>NNCPLDWLPMNGLCYKIFNQLKTWEDAEMFCRKYKPGCHLASFHRYGESLEIAEYISDYHKGQENVWIGLRDKKKDFSWEWTDRSCTDYLTWDKNQPDHYQNKEF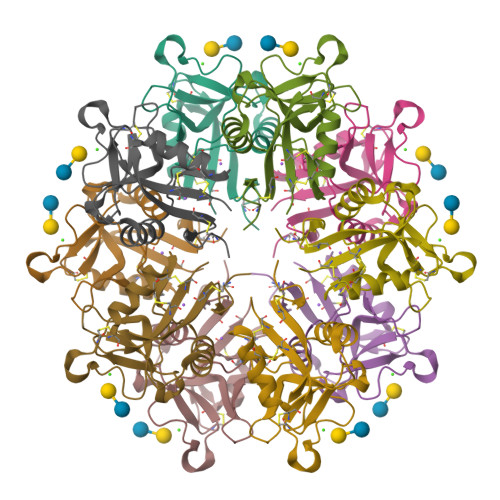CVELVSLTGYRLWNDQVCESKDAFLCQCKF[5x]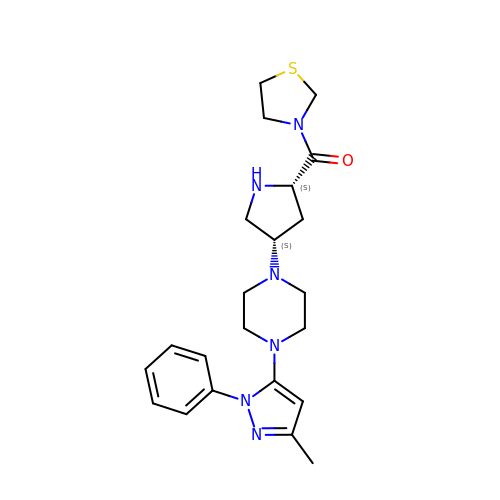{(2S,4S)-4-[4-(3-methyl-1-phenyl-1H-pyrazol-5-yl)piperazin-1-yl]pyrrolidin-2-yl}(1,3-thiazolidin-3-yl)methanone | C22 H30 N6 O S | WGRQANOPCQRCME-PMACEKPBSA-N> GPLGSMAFLAQLGALADDLVSAIVGIPEDQTTQRDACRDFVLRSLRHHNFGRTNQFEVQDRLNGLEERFSIVGRDALADALRTRLDALEPHQNQFTPELLHLLLELADQ;> GPHMPPSERAEKQAAA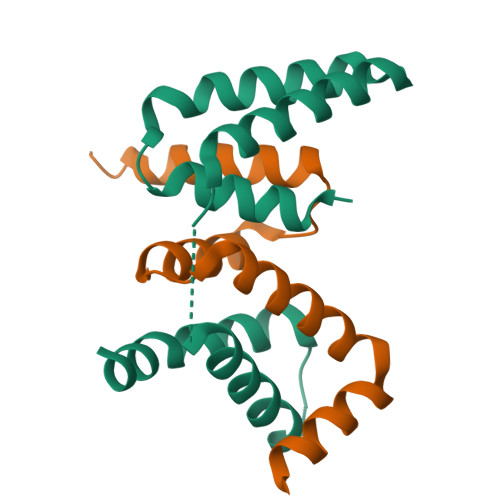QQAVDILHEIATILNCHLDRRTLSICISMIENGVNPEALANVIKELRVLGQDPQQLDALVANYLASSRRR> MAYAQWVIIIIHNVGSQDVKIKNLKASWGKLHADGDKDAEVSASNYEGKIVKPDEKLQINASGRSDAAEGTTGTFDLVDPADGDKQVRHFYWDSPWGSKTNTWTVSGSNTKWMIEYSGQNLDSGALGTITVDTLKKGENLY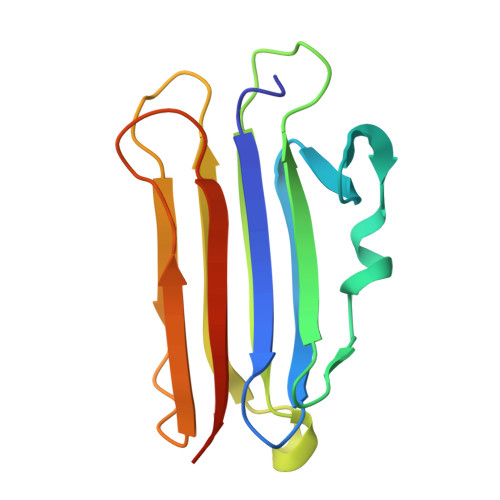FQ>GPGSMVVAVDGPSGTGKSSVAKELARQLGASYLDTGAMYRIVTLWVLRAGVDLTDPAAIAAATDQVPMSVSSDPDAQTALLAGEDVSVPIRGNEVTGAVSAVSAVPAVRERLVRQQRELAESSGAVVVEGRDIGTVVLPDADVKIYLTASAQARAQRRNAQNVSGGGDDEYEKVLADVQRRDHLDSTRAVSPLRPAEDALEVDTSDMTQEQVVAHLLDLVRTRAGASR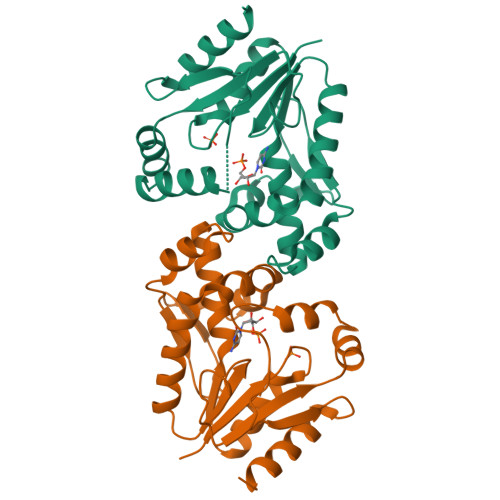[4x]> TWQWVLINISEEARQLIEKAVRAISKKEGTEVHFEKDDGVLH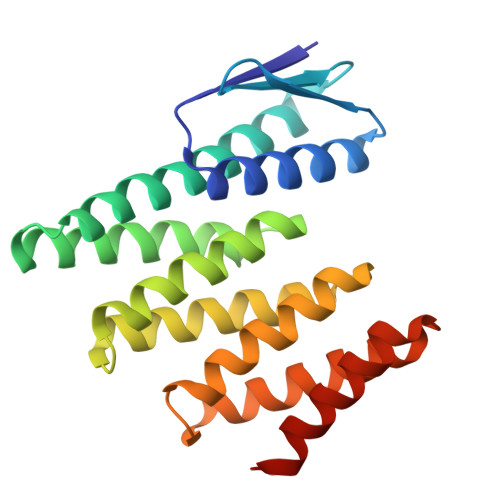IRVKNLHEKRAREIHKVAKLILEVAAAERIVRERPGSNLAKKALEIILRAAEELAKADVDAALEAAVRAAEKVVREQPGSNLAKKALEIILRAAEELAKLPDPEALKEAVKAAEKVVREQPGSELAKKALEIIERAAEELKKSPDPEAQKEAKKAEQKVREERPGS>[2x]TDQPECYKITYPKPLYSSSVPANYSDPQFAVAVCNNYLHENYPTVASYQITDEYDAYLDMVDGTVACLDTATFSPAKLRSYPKKHEYRAPNIRSAVPSAMQNTLQNVLIAATKRNCNVTQMRELPTLDSATFNVECFRKYA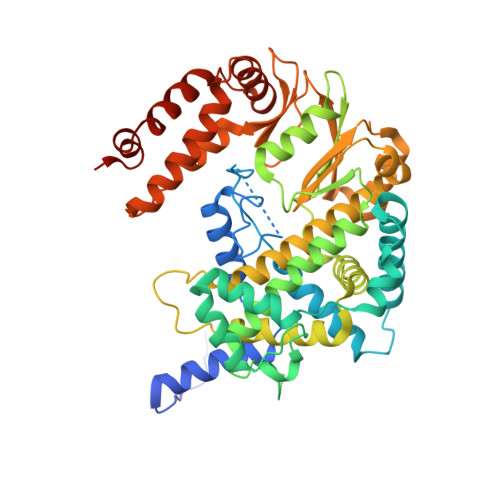CNDEYWEEFARKPIRITTEFVTAYVARLKGPKAAALFAKTYNLVPLQEVPMDRFVMDMKRDVKVTPGTKHTEERPKVQVIQAAEPLATAYLCGIHRELVRRLTAVLLPNIHTLFDMSAEDFDAIIAEHFKQGDPVLETDIASFDKSQDDAMALTGLMILEDLGVDQPLLDLIECAFGEISSTHLPTGTRFKFGAMMKSGMFLTLFVNTVLNVVIASRVLEERLKTSRCAAFIGDDNIIHGVVSDKEMAERCATWLNMEVKIIDAVIGERPPYFCGGFILQDSVTSTACRVADPLKRLFKLGKPLPADDEQDEDRRRALLDETKAWFRVGITGTLAVAVTTRYEVDNITPVLLALRTFAQSKRAFQAIRGEIKHLYGGPK> MLKSRVILAMDKPLSYQVLKEMENELYGIKVGLPLVLDLGVDKTRELLIGLDV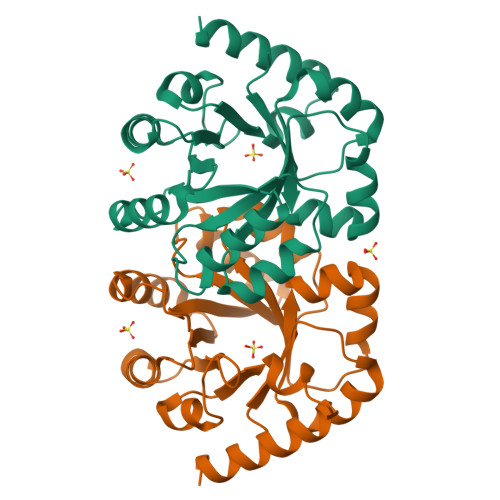EEIIVDFKLADIGYIMKSIVERLSFANSFIAHSFIGVKGSLDELKRYLDANSKNLYLVAVMSHEGWSTLFADYIKNVIREISPKGIVVGGTKLDHITQYRRDFEKMTIVSPGMGSQGGSYGDAVCAGADYEIIGRSIYNAGNPLTALRTINKIIEDKVMKCKGAIFRKK>RLKKRIFAAVSEGCVEELRELLQDLQDLCRRRRGLDVPDFLMHKLTASDTGKTCLMKALLNINPNTKEIVRILLAFAEENDILDRFINAEYTEEAYEGQTALNIAIERRQGDITAVLIAAGADVNAHAKGVFFNPKYQHEGFYFGETPLALAACTNQPEIVQLLMENEQTDITSQDSRGNNILHALVTVAEDFKTQNDFVKRMYDMIL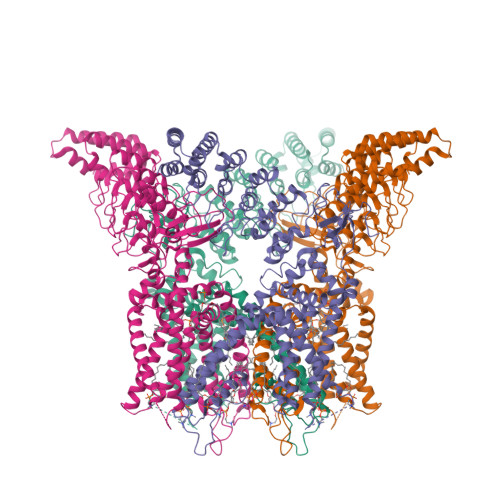LRSGNWELETMRNNDGLTPLQLAAKMGKAEILKYILSREIKEKPLRSLSRKFTDWAYGPVSSSLYDLTNVDTTTDNSVLEIIVYNTNIDNRHEMLTLEPLHTLLHTKWKKFAKYMFFLSFCFYFFYNITLTLVSYYRPREDEDLPHPLALTHKMSWLQLLGRMFVLIWATCISVKEGIAIFLLRPSDLQSILSDAWFHFVFFVQAVLVILSVFLYLFAYKEYLACLVLAMALGWANMLYYTRGFQSMGMYSVMIQKVILHDVLKFLFVYILFLLGFGVALASLIEKCSKDKKDCSSYGSFSDAVLELFKLTIGLGDLNIQQNSTYPILFLFLLITYVILTFVLLLNMLIALMGETVENVSKESERIWRLQRARTILEFEKMLPEWLRSRFRMGELCKVADEDFRLCLRINEVKWTEWKTHVSFLNEDPGPI[4x]>MAKRLSKQQLAKAIANTLETPPQPKAGRRRNRRRQRSAVQQLQPTQAGISMAPSAQGAMVRIRNPAVSSSRGGITVLTHSELSAEIGVTDSIVVSSELVMPYTVGTWLRGVAANWSKYSWLSVRYT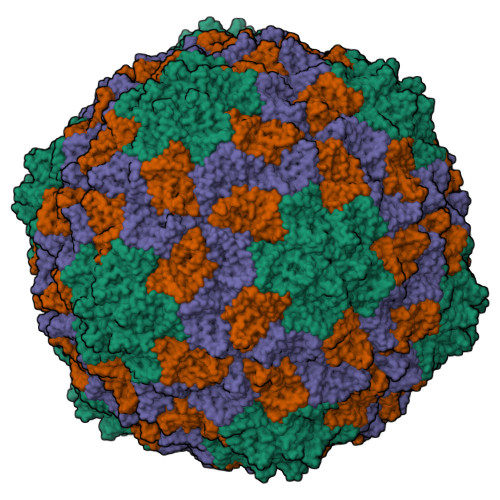YIPSCPSSTAGSIHMGFQYDMADTVPVSVNQLSNLRGYVSGQVWSGSAGLCFINGTRCSDTSTAISTTLDVSKLGKKWYPYKTSADYATAVGVDVNIATPLVPARLVIALLDGSSSTAVAAGRIYCTYTIQMIEPTASALNN[3x]> SAKDERAREILRGFKLNWMNLRDAETGKILWQGTEDLSVPGVEHEARVPKKILKCKAVSRELNFSSTEQMEKFRLEQKVYFKGQCLEEWFFEFGFVIPNSTNTWQSLIEAAPESQMMPASVLTGNVIIETKFFDD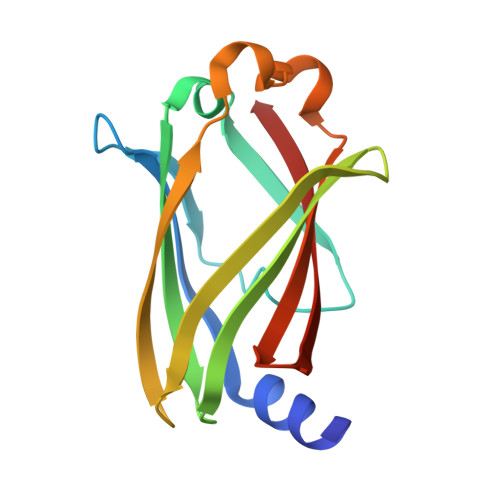DLLVSTSRVRLFYV> YKKALKKL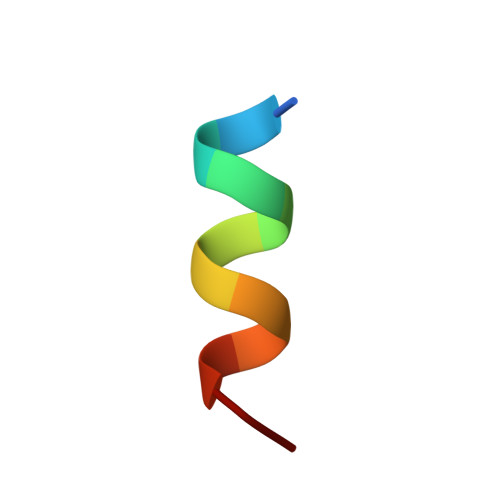AKLL Glutaminase catalyzes the first step of glutamine metabolism, converting glutamine to glutamate, which enters the tricarboxylic acid cycle. In human, glutaminase is encoded by two different genes, GLS1 and GLS2.1 GLS1 can be alternatively spliced into kidney glutaminase A (KGA) and highly active glutaminase isoform C (GAC)1. Glutaminase, especially the GAC isoform, is highly overexpressed in various cancers for the utilization of glutamine. GAC can be further activated by anions. It has been observed that GAC can form active filaments both in vitro and in vivo.

We resolved the structure of GAC filament at a resolution of 2.9 Å. GAC forms filaments with tetramers as the helical unit. The helical assembly interface is composed of four protomers. The secondary structures involved in the assembly interface are α-helices 351–365, 375–384, 407–419 and β-barrel 371–373. Sequence alignment shows that the amino acids involved in the helical interface, F355, F373, N375, F378, Q379, and Q416, are highly conserved in mammalian glutaminase. To investigate the functional significance of GAC filamentation and its relationship with Pi, we designed point mutations disrupting the filamentation interface of GAC. Negative-stain electron microscopy (EM) revealed that Q416A disrupted the filamentation of GAC. We then performed activity assays on Q416A. In the Apo state and the Pi bound state, the activities of Q416A are 0.26 times and 0.63 times of those of the wild-type GAC, respectively. In the highly active filament, the helical interface is located on the catalytic core of GAC, and the tetramers are compressed.

>[4x]LVASGENKIKQGLLPSLEDLLFYTIAEGQEKIPVHKFITALKSTGLRTSDPRLKECMDMLRLTLQTTSDGVMLDKDLFKKCVQSNIVLLTQAFRRKFVIPDFMSFTSHIDELYESAKKQSGGKVADYIPQLAKFSPDLWGVSVCTVDGQRHSTGDTKVPFCLQSCVKPLKYAIAVNDLGTEYVHRYVGKEPSGLRFNKLFLNEDDKPHNPMVNAGAIVVTSLIKQGVNNAEKFDYVMQFLNKMAGNEYVGFSNATFQSERESGDRNFAIGYYLKEKKCFPEGTDMVGILDFYFQLCSIEVTCESASVMAATLANGGFCPITGERVLSPEAVRNTLSLMHSCGMYDFSGQFAFHVGLPAKSGVAGGILLVVPNVMGMMCWSPPLDKMGNSVKGIHFCHDLVSLCNFHNYDNLRHFAKKLDPRREGGDQRHSFGPLDYESLQQELALKETVWKKVSPESNEDISTTVVYRMESLGEKS>[3x]SKTIVLSVGEATRTLTEIQSTADRQIFEEKVGPLVGRLRLTASLRQNGAKTAYRVNLKLDQADVVDCSTSVC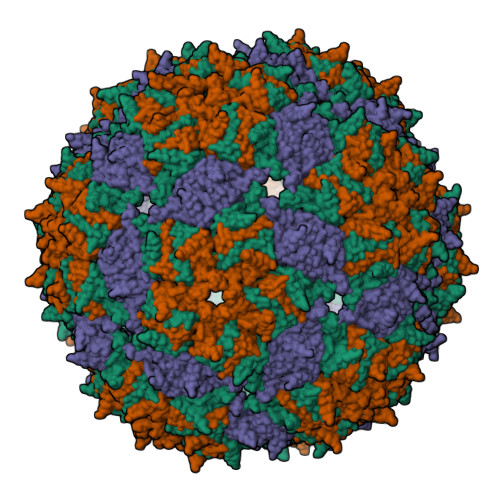GELPKVRYTQVWSHDVTIVANSTEASRKSLYDLTKSLVATSQVEDLVVNLVPLGR>VSPIIATILLIAITVVLAATLVTILGGFTHGVSNTVETAGVTSHITSKYIFINVSSSSSAISASSITITITGASFKVTSGDTLAEVAGVSSTSSNATFTGGSDYTVPISLSSSQTVAGVSFELIYKGNVIYNSAA[36x]

Archaeal Type IV pilins and archaellins, which form the subunits of pili and archaella, respectively, are expressed as preproteins with a signal peptide. The pilins/archaellins are then assembled into a filament, wherein the hydrophobic alpha helical N-termini are helically stacked in the core of the filament, and the hydrophilic β-strand-rich heads are oriented towards the filament's periphery. Through single particle cryo-electron microscopy (cryoEM) and helical reconstruction, we solved the structures of these filaments at 2.61 and 2.52 Å resolution for C. divulgatum and O. meridianum, respectively. Atomic model building, bioinformatics analysis, and motility experiments suggest that the C. divulgatum fibre is a nonrotary, likely adhesive T4P, whereas the O. meridianum filament is an archaellum.

We will henceforth name the filament of C. divulgatum pilus (CdiP), and, by applying the same nomenclature system as for the genes of the homologous S. acidocaldarius, we will refer to its subunit pilin as CdiPB. The protein is 135 residues long and folds into an N-terminal α-helical tail, followed by a globular head. The FlaFind server, determined a class-III peptidase cleavage site between residues 11 and 12, indicating that the first 11 residues are proteolytically removed during the maturation of the protein, as is typical for Type-IV pilins The head domain is composed of six β-strands that fold into two β-sheets but unusually also contains three short α-helices (α2, α3, and α4). In addition, CdiPB contains a comparatively long linker region of 12 amino acids between the head and the tail of the protein (G38 to A50). When building the atomic model for CdiPB, we identified two N-linked glycans for each subunit, originating from conserved NXS/T sequons (N64 and N106). The densities for the two glycosylation sites were well resolved, allowing the assignment of six and five sugars for N64 and N106, respectively. In each of its three component helices, AapB adopts a unique conformation, distinguished by the angle between the head and the tail domain, as well as the structure of the hinge. Such a three-conformer architecture is not evident in the CdiP pilus. In contrast to the twitching Aap of S. acidocladarius, the CdiP does not have the distinct three-conformer structure that has been proposed to aid the collapse of the Aap into the membrane during twitching motility, and indeed, we were unable to detect twitching motility in C. divulgatum. It follows that the long hinge may have evolved to provide the CdiP filament with particularly high degrees of flexibility, which may aid surface adhesion, cell–cell contacts, and biofilm formation. The cells mainly adhered to the surface of the substrate but did not display twitching motility.>[3x]MSRKNISLTESLEEYIFRNSVREPDSFLKLRKETGTLAQANMQISPEEGQFLNILTKISGAKRIIEIGTFTGYSSLCFASALPEDGKI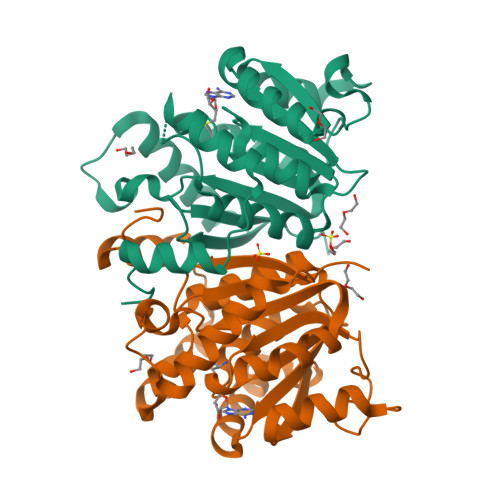LCCDVSEEWTNVARKYWKENGLENKIFLKLGSALETLQVLIDSKSAPSWASDFAFGPSSIDLFFLDADKENYPNYYPLILKLLKPGGLLIADNVLWDGSVADLSHQEPSTVGIRKFNELVYNDSLVDVSLVPIADGVSLVRKRLEHHHHHH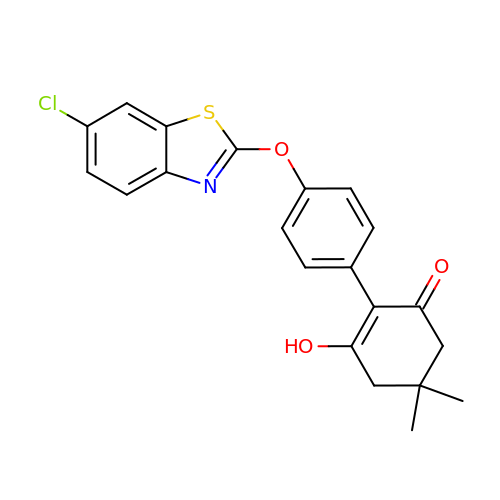4'-[(6-chloro-1,3-benzothiazol-2-yl)oxy]-6-hydroxy-4,4-dimethyl-4,5-dihydro[1,1'-biphenyl]-2(3H)-one | C21 H18 Cl N O3 S | POUJNUFBEAPAJW-UHFFFAOYSA-N> MLRFTQVIRKNPVVFKQGQGMFSHQLKRILNKK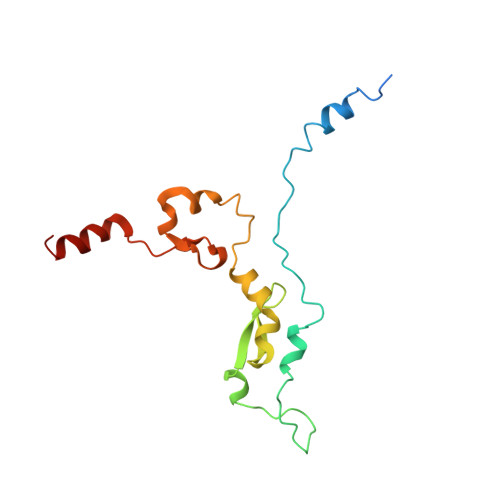SLHKYNWDPLHMYDPRKLVHANRYVDHDTYEEKYDPHWEHNAHLVPDQQFYNIPVPKEYKDAYWWRDLQARRVQCPTEWVHFRMHTKDKLKYDFQDLAFRKKFEYSYEDVVANAKDMCS>[2x]MQPINTSNPDNTASYVKDEVEITSSTIALSEIVSVVNTSDGRLEVFGVGTDKAVWHNRQMAPHTGSPWSGWSSLKGQVTSKPVVYINTDGRLEVFARGTDNALWHIWQTATNAGWSNWQSLGGVITSNPAIYANTDGRLEVFARGADNALWHISQTTAHSGPWSSWASLNGVITSNPTVHINSDGRLEVFARGTDNALWHIWQTAPDSNLWSSWESLNGIITSDPVVIDTADGRLEVFARGADNALWHIWQTISHSGPWSGWQSLNGVITSAPAVAKNCDNRLEAFARGTDNALWHTWQTVSHSGPWSSWQSLNGVITSAPTAVRDADGRLEVFARGTDNALWLTWQTASSWSPWISLGGVLIDASAIK

As a part of our ongoing programme focused on host-pathogen interactions at the molecular level, we identified a lectin in the P. asymbiotica genome designated PHL, which we prepared in a fully functional recombinant form. The lectin PHL interacts selectively, mainly with l-fucose and oligosaccharides containing terminal l-fucose residue, and prefers an α-glycosidic bond over a β-linkage. The PHL lectin forms a seven-bladed β-propeller assembling into a homo-dimer. Both units contain two types of binding sites situated between the blades and have different amino acid compositions and binding preferences.

As mixing PHL with the branched compounds leads to protein precipitation and thus prevents co-crystallization, the direct study of complexes was not possible. Therefore, we soaked the PHL crystals with monomeric fucoside 2, 3 and 4, respectively. Crystal structures confirmed that all the studied fucosides were able to bind the lectin PHL. In each complex, the electron density was clear enough to determine the position of the fucosyl part of the compounds in 6 out of 7 fucose-binding sites of at least one PHL monomer unit – A or B, while site 2 is occupied by Met60 of the neighbouring monomer, as was observed previously. The second saccharide unit was clearly assigned for all three fucosides 2–4 in sites 1 and 3. Considering fucosides 2–4, the position of the bridging methylene group is close to the α-Me-Fuc O1 atom, which is not directly coordinated by the protein in the complex. The O4 of the d-arabino-hexopyranosyl unit in fucoside 2 and 4 is coordinated by a glycine backbone nitrogen in sites 1, 3, 5, and 6, while the O6 atom of fucoside 3 is linked to a tryptophan backbone oxygen in sites 4 and 6. When comparing the overall orientation of the second hexopyranosyl unit of fucosides 2–4, it is similar to the galactose unit of blood group H trisaccharide, with minor distortions in individual binding sites influenced e.g. by crystal packing. The remaining parts of fucosides 2 and 3 were not resolved in the electron density, suggesting their negligible importance for ligand binding. The second saccharide unit of studied fucosides was only marginally coordinated by PHL binding sites what, together with affinity comparable to monosaccharides, suggests a low importance of this type of compounds for inhibitor design.>[2x]MEFKKVAKETAITLQSYLTYQAVRLISQQLSETNPGQAIWLGEFSKRHPI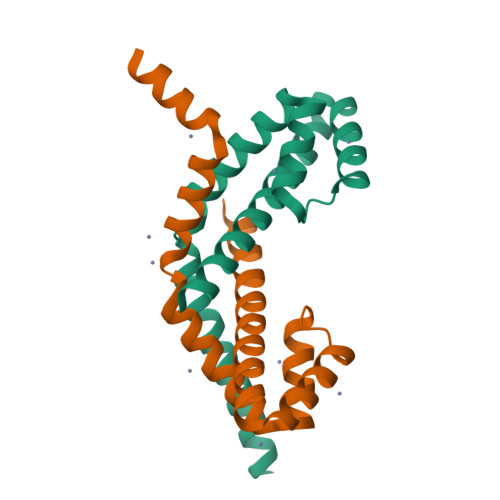QESDLYLEAMMLENKELVLRILTVRENLAEGVLEFLPEMVLSQIKQSNGNHRRSLLERLTQVDSSSTDQTEPNPGESDTSEDSE> RNILMNDEGLYAGQSLDVEPYHLIMQEDCNLVLYDHSTAVWTTNTDIPGKKGCKAVLQSDGNFVVYDAEGRSLWASHSV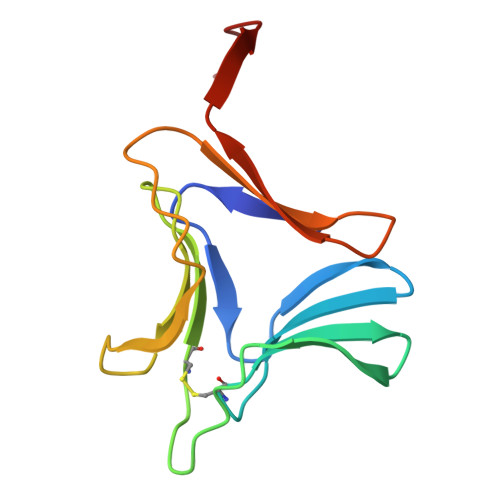RGNGNYVLVLQEDGNVVIYGSDIWSTNTYK> GNYMGNPWTEYMAKYDIEEVHGSGIRVDLGEDAE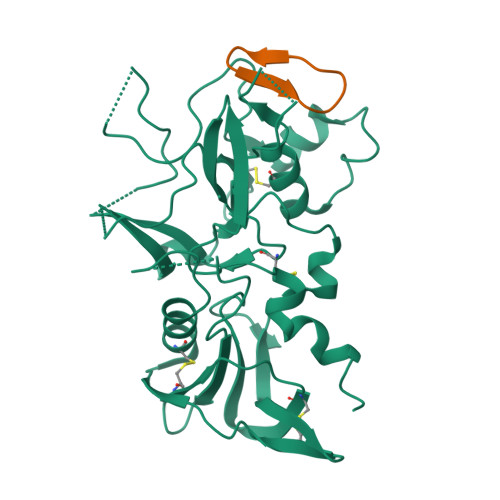VAGTQYRLPSGKCPVFGKGIIIENSNTTFLKPVATGNQDLKDGGFAFPPTNPLISPMTLNGMRDFYKNNEYVKNLDELTLCSRHAGNMNPDNDKNSNYKYPAVYDYNDKKCHILYIAAQENNGPRYCNKDESKRNSMFCFRPAKDKLFENYTYLSKNVVDNWEEVCPRKNLENAKFGLWVDGNCEDIPHVNEFSANDLFECNKLVFELSASDQPKQYEQHLTDYEKIKEGFKNKNASMIKSAFLPTGAFKADRYKSHGKGYNWGNYNRETQKCEIFNVKPTCLINNSSYIATTALSHPIEVE;> CWTTRMSPPMQIP>[2x]ACPEDWGASSRTSLCFKLYAKGKHEKKTWFESRDFCRALGGDLASINNKEEQQTIWRLITASGSYHKLFWLGLTYGSPSEGFTWSDGSPVSYENWAYGEPNNYQNVEYCG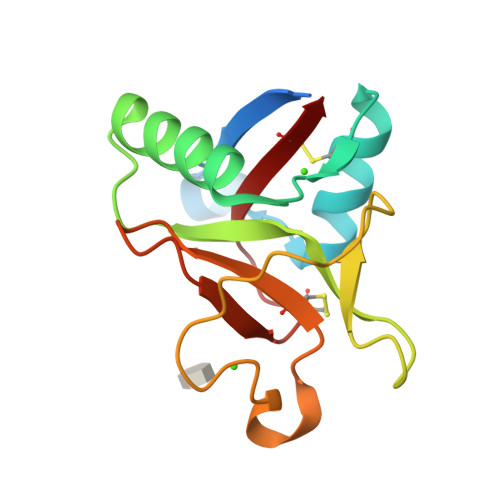ELKGDPTMSWNDINCEHLNNWICQI>MMQQSRPASDPQVVEAARKEGRLIIYSSTAQSSAQALLDDFRKLYPFIQIEYNDLGTQAIYDRFVSETAAGASSADLLWSSAMELQVKLASEGYALPYDSPEAKNWPANARLGNLAYSTTLEPAVVVYNKRFLKPEEVPTTREGLARLLQEPRMRGRVATWDPERSAVGFTILKADYDRFPAFQELARAFGKAQAALYSSTGAAFEKVISGEHYLAYGFFGSYALLRQRTVKDLGIAYLTDGTVAIQRVAFINKRAAHPNAAKLFLDYLLSLRGQNLMAYTALIFARRETVVGEATPQALYKAVGGKDKVYAIPVSTEILKNLDPAERMRF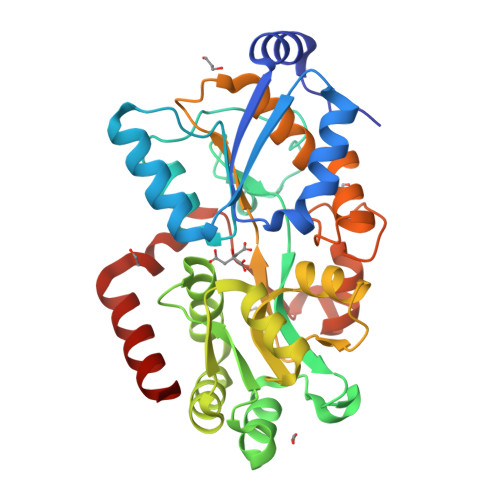LTFWRQAVRGQ[3x]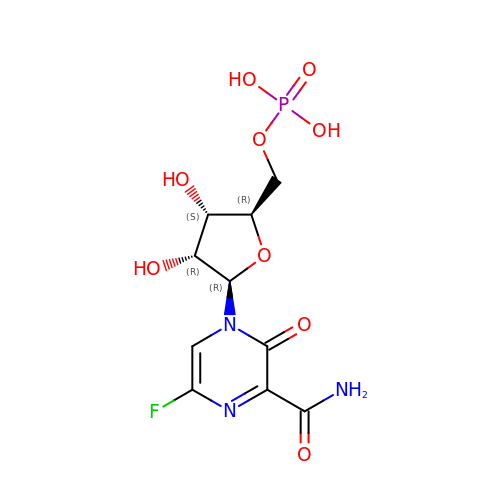6-fluoro-3-oxo-4-(5-O-phosphono-beta-D-ribofuranosyl)-3,4-dihydropyrazine-2-carboxamide | C10 H13 F N3 O9 P | RWCWUNIDADUVEZ-KAFVXXCXSA-N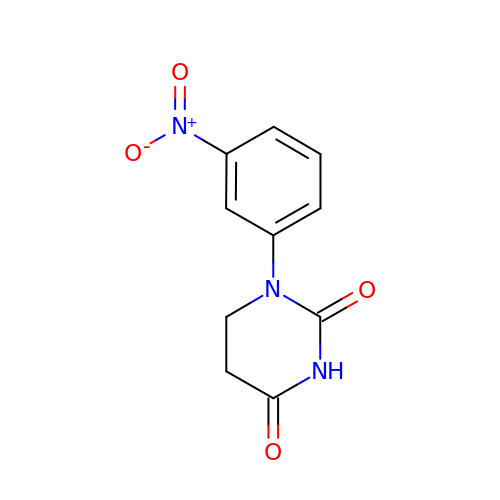1-(3-nitrophenyl)dihydropyrimidine-2,4(1H,3H)-dione | C10 H9 N3 O4 | GMUGBPYYXAGNCT-UHFFFAOYSA-N> GPVDPKMLRWPLRFVIGSSDTQRSLLGRIGIGDVLLIRTSRAEVYCYAKKLGHFNRVEGGIIVETLDIQHIEE;> GPVDVKLEFVLYRKNVTLAELEAMGQQQLLSLPTNAELNV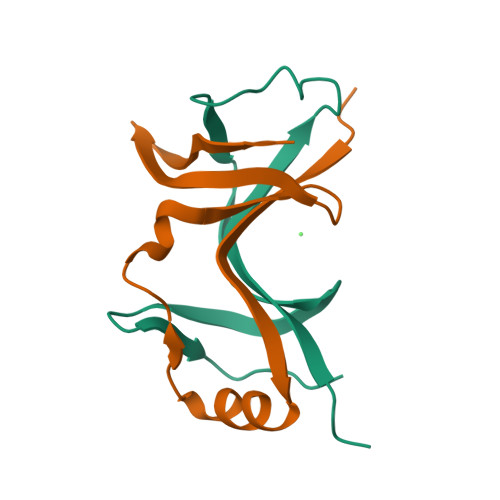EIMANGVLLGNGELVQMNDTLGVEIHEWLS>[7x]YLVPTVIEQSG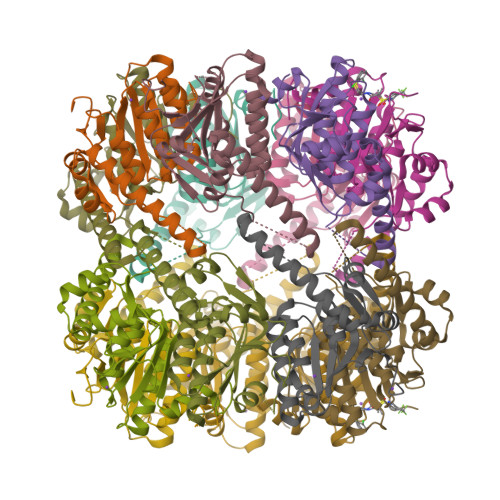RGERAFDIYSRLLKERIVFLVGPVTDESANLVVAQLLFLESENPDKDIFFYINSPGGSVTAGMSIYDTMNFIKPDVSTLCLGQAASMGAFLLSAGEKGKRFALPNSRIMIHQPLISGGLGGQASDIEIHARELLKIKEKLNRLMAKHCDRDLADLERDTDRDNFMSAEEAKEYGLIDQILENRASLRL>[2x]MALSTATKAATDALAANRAPTSVNAQEVHRWLQSFNWDFKNNRTKYATKYKMANETKEQFKLIAKEYARMEAVKDERQFGSLQDALTRLNAGVRVHPKWNETMKVVSNFLEVGEYNAIAATGMLWDSAQAAEQKNGYLAQVLDEIRHTHQCAYVNYYFAKNGQDPAGHNDARRTRTIGPLWKGMKRVFSDGFISGDAVECSLNLQLVGEACFTNPLIVAVTEWAAANGDEITPTVFLSIETDELRHMANGYQTVVSIANDPASAKYLNTDLNNAFWTQQKYFTPVLGMLFEYGSKFKVEPWVKTWDRWVYEDWGGIWIGRLGKYGVESPRSLKDAKQDAYWAHHDLYLLAYALWPTGFFRLALPDQEEMEWFEANYPGWYDHYGKIYEEWRARGCEDPSSGFIPLMWFIENNHPIYIDRVSQVPFCPSLAKGASTLRVHEYNGEMHTFSDQWGERMWLAEPERYECQNIFEQYEGRELSEVIAELHGLRSDGKTLIAQPHVRGDKLWTLDDIKRLNCVFKNPVKAFN;>MSMLGERRRGLTDPEMAAVILKALPEAPLDGNNKMGYFVTPRWKRLTEYEALTVYAQPNADWIAGGLD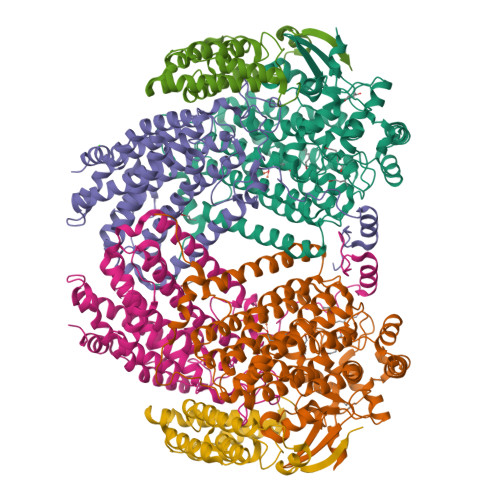WGDWTQKFHGGRPSWGNETTELRTVDWFKHRDPLRRWHAPYVKDKAEEWRYTDRFLQGYSADGQIRAMNPTWRDEFINRYWGAFLFNEYGLFNAHSQGAREALSDVTRVSLAFWGFDKIDIAQMIQLERGFLAKIVPGFDESTAVPKAEWTNGEVYKSARLAVEGLWQEVFDWNESAFSVHAVYDALFGQFVRREFFQRLAPRFGDNLTPFFINQAQTYFQIAKQGVQDLYYNCLGDDPEFSDYNRTVMRNWTGKWLEPTIAALRDFMGLFAKLPAGTTDKEEITASLYRVVDDWIEDYASRIDFKADRDQIVKAVLAGLK[2x];>[2x]MAKLGIHSNDTRDAWVNKIAQLNTLEKAAEMLKQFRMDHTTPFRNSYELDNDYLWIEAKLEEKVAVLKARAFNEVDFRHKTAFGEDAKSVLDGTVAKMNAAKDKWEAEKIHIGFRQAYKPPIMPVNYFLDGERQLGTRLMELRNLNYYDTPLEELRKQRGVRVVHLQSPH>MRGSHHHHHHGSMKVWLDGRLVDEEEAKVTVLSPSLNYGFGVFEGIRAYWNGENLYVFRLRDHMERLLRSAKIIGLDVPYTAEELSKAVVETVRANGFKEDLYIRPVAYISKPQISLDVRGLQASVAIAAIPFGKYLKVEGVRAAVVSWRRVHTSMMPVMAKATGIYLNSIMAAVEARARGYDEAIMLNAEGKVVEGSGENIFIVRRGVLMTPPLEDGILEGITRETVISIAGDLGIPLLEKSITREELYAADEAFFV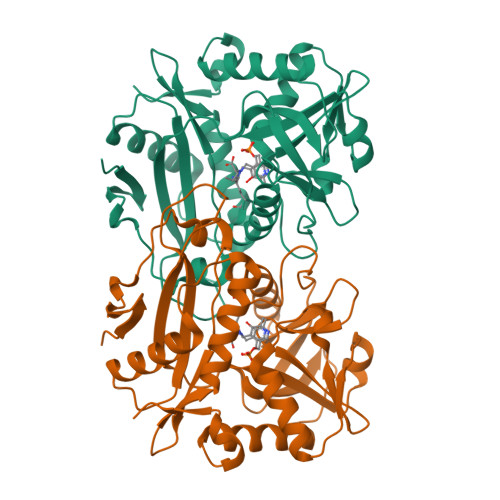GTAAEITPIIEIDGRVLQRGPITQKIAETYRRIVLGKEEKYLPWLTPVY[3x]> MRVGIPTETKNNEFRV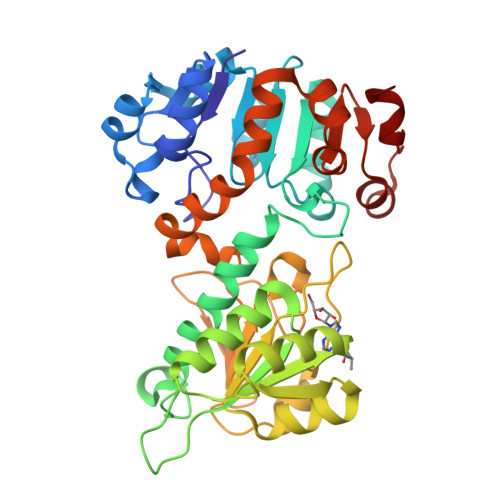AITPAGVAELTRRGHEVLIQAGAGEGSAITDADFKAAGAQLVGTADQVWADADLLLKVKEPIAAEYGRLRHGQILFTFLHLAASRACTDALLDSGTTSIAYETVQTADGALPLLAPMSEVAGRLAAQVGAYHLMRTQGGRGVLMGGVPGVEPADVVVIGAGTAGYNAARIANGMGATVTVLDINIDKLRQLDAEFCGRIHTRYSSAYELEGAVKRADLVIGAVLVPGAKAPKLVSNSLVAHMKPGAVLVDIAIDQGGCFEGSRPTTYDHPTFAVHDTLFYCVANMPASVPKTSTYALTNATMPYVLELADHGWRAACRSNPALAKGLSTHEGALLSERVATDLGVPFTEPASVLA>MMVISEKVRKALNDQLNREIYSSYLYLSMATYFDAEGFKGFAHWMKKQAQEELTHAMKFYEYIYERGGRVELEAIEKPPSNWAGIKDAFEAALKHEEFVTQSIYNILELASEEKDHATVSFLKWFVDEQVEEEDQVREILDLLEKAYGQMSV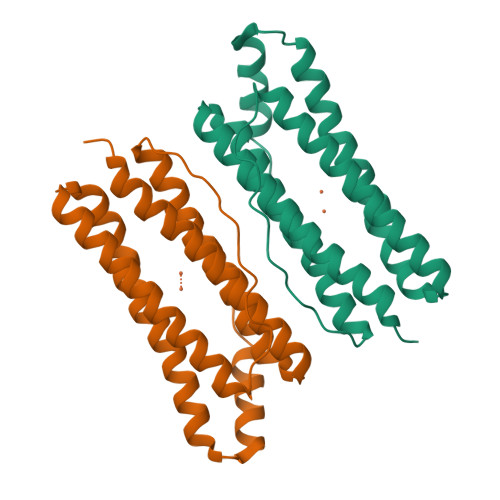IFQLDRYLGQRE[4x]> GSNGMSQLPAPVSVESSWRYIDTQGQIHGPFTT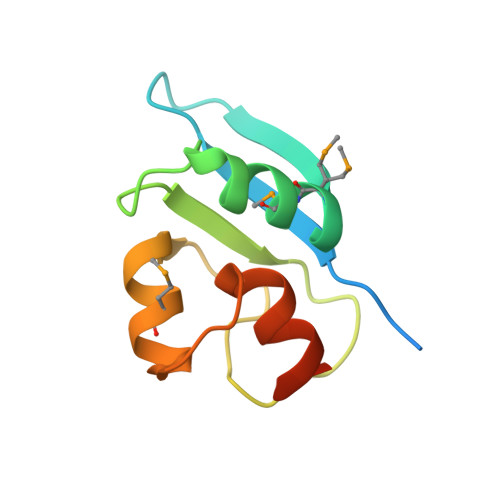QMMSQWYIGGYFASTLQISRLGSTPETLGINDIFITLGELMTKLEKYDTDPFTTFDKLHVQTTSSDS> MLPVYQEVKPNPLQDANLCSRVFFWWLNPLFKIGHKRRLEEDDMYSVLPEDRSQHLGEELQGFWDKEVLRAENDAQKPSLTRAIIKCYWKSYLVLGIFTLIEESAKVIQPIFLGKIINYFENYDPMDSVALNTAYAYATVLTFCTLILAILHHLYFYHVQCAGMRLRVAMCHMIYRKALRLSNMAMGKTTTGQIVNLLSNDVNKFDQVTVFLHFLWAGPLQAIAVTALLWMEIGISCLAGMAVLIILLPLQSCFGKLFSSLRSKTATFTDARIRTMNEVITGIRIIKMYAWEKSFSNLITNLRKKEISKILRSSCLRGMNLASFFSASKIIVFVTFTTYVLLGSVITASRVFVAVTLYGAVRLTVTLFFPSAIERVSEAIVSIRRIQTFLLLDEISQRNRQLPSDGKKMVHVQDFTAFWDKASETPTLQGLSFTVRPGELLAVVGPVGAGKSSLLSAVLGELAPSHGLVSVHGRIAYVSQQPWVFSGTLRSNILFGKKYEKERYEKVIKACALKKDLQLLEDGDLTVIGDRGTTLSGGQKARVNLARAVYQDADIYLLDDPLSAVDAEVSRHLFELCICQILHEKITILVTHQLQYLKAASQILILKDGKMVQKGTYTEFLKSGIDFGSLLKKDNEESEQPPVPGTPTLRNRTFSESSVWSQQSSRPSLKDGALESQDTENVPVTLSEENRSEGKVGFQAYKNYFRAGAHWIVFIFLILLNTAAQVAYVLQDWWLSYWANKQSMLNVTVNGGGNVTEKLDLNWYLGIYSGLTVATVLFGIARSLLVFYVLVNSSQTLHNKMFESILKAPVLFFDRNPIGRILNRFSKDIGHLDDLLPLTFLDFIQTLLQVVGVVSVAVAVIPWIAIPLVPLGIIFIFLRRYFLETSRDVKRLESTTRSPVFSHLSSSLQGLWTIRAYKAEERCQELFDAHQDLHSEAWFLFLTTSRWFAVRLDAICAMFVIIVAFGSLILAKTLDAGQVGLALSYALTLMGMFQWCVRQSAEVENMMISVERVIEYTDLEKEAPWEYQKRPPPAWPHEGVIIFDNVNFMYSPGGPLVLKHLTALIKSQEKVGIVGRTGAGKSSLISALFRLSEPEGKIWIDKILTTEIGLHDLRKKMS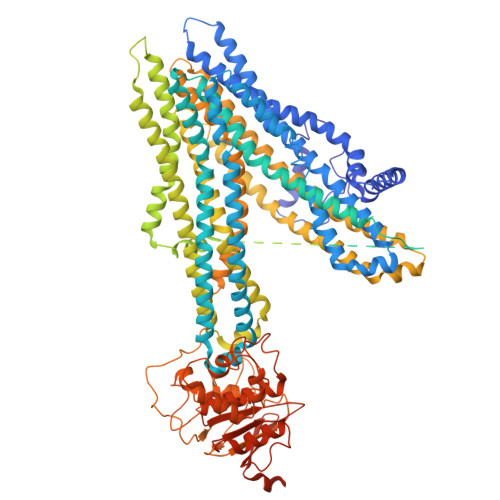IIPQEPVLFTGTMRKNLDPFNEHTDEELWNALQEVQLKETIEDLPGKMDTELAESGSNFSVGQRQLVCLARAILRKNQILIIDEATANVDPRTDELIQKKIREKFAHCTVLTIAHRLNTIIDSDKIMVLDSGRLKEYDEPYVLLQNKESLFYKMVQQLGKAEAAALTETAKQVYFKRNYPHIGHTDHMVTNTSNGQPSTLTIFETAL>[2x]SMFNVSNNVAPSRYQGPSSTSVTPNA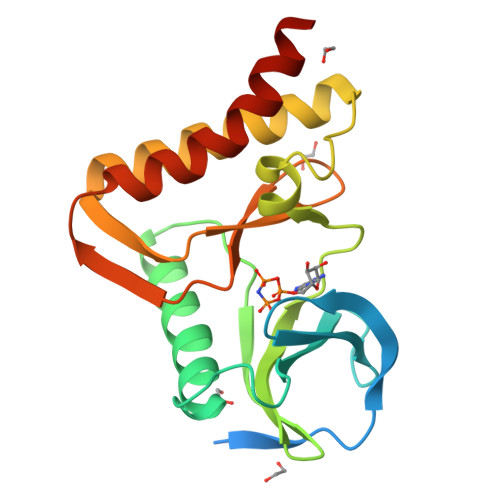FHDVPSLGQKVGAGSQKDVFHSRQDPRQCICLFRPGTTGSIPAEQYAQKELETTKQLKNLGFPVVDAHALVKHQGSVGVAKDFIHNALDSEDIVNNKKSLPDNLKFNKNVLEDCNAIIRRLKNLEVHIEDLQFLVDHNGHVLINDPRDVVRSSPDKSISKVNELRSHALNNLLDIDSD>[2x]MGLLLPLALCILVLCCGAMSPPQLALNPSALLSRGCNDSDVLAVAGFALRDINKDRKDGYVLRLNRVNDAQEYRRGGLGSLFYLTLDVLETDCHVLRKKAWQDCGMRIFFESVYGQCKAIFYMNNPSRVLYLAAYNCTLRPVSKKKIYMTCPDCPSSIPTDSSNHQVLEAATESLAKYNNENTSKQYSLFKVTRASSQWVVGPSYFVEYLIKESPCTKSQASS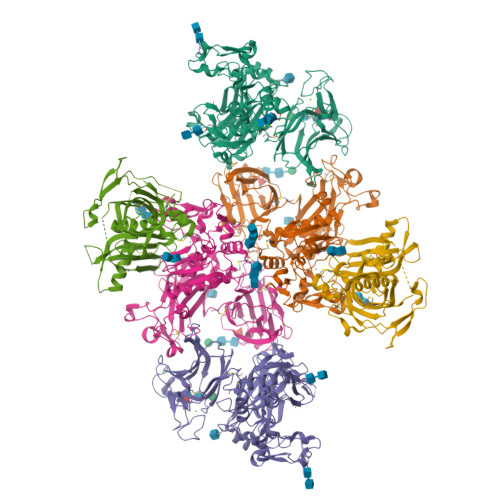CSLQSSDSVPVGLCKGSLTRTHWEKFVSVTCDFFESQAPATGSENSAVNQKPTNLPKVEESQQKNTPPTDSPSKAGPRGSVQYLPDLDDKNSQEKGPQEAFPVHLDLTTNPQGETLDISFLFLEPMEEKLVVLPFPKEKARTAECPGPAQNASPLVLPPHHHHHH;>WSHPQFEKVPIKYLPEENVHDADFGEQKDISEINLAAGLDLFQGDILLQKSRNGLRDPNTRWTFPIPYILADNLGLNAKGAILYAFEMFRLKSCVDFKPYEGESSYIIFQQFDGCWSEVGDQHVGQNISIGQGCAYKAIIEHEILHALGFYHEQSRTDRDDYVNIWWDQILSGYQHNFDTYDDSLITDLNTPYDYESLMHYQPFSFNKNASVPTITAKIPEFNSIIGQRLDFSAIDLERLNRMYNCTTTHTLLDHCTFEKANICGMIQGTRDDTDWAHQDSAQAGEVDHTLLGQCTGAGYFMQFSTSSGSAEEAALLESRILYPKRKQQCLQFFYKMTGSPSDRLVVWVRRDDSTGNVRKLVKVQTFQGDDDHNWKIAHVVLKEEQKFRYLFQGTKGDPQNSTGGIYLDDITLTETPCPTGVWTVRNFSQVLENTSKGDKLQSPRFYNSEGYGFGVTLYPNSRESSGYLRLAFHVCSGENDAILEWPVENRQVIITILDQEPDVRNRMSSSMVFTTSKSHTSPAINDTVIWDRPSRVGTYHTDCNCFRSIDLGWSGFISHQMLKRRSFLKNDDLIIFVDFEDITHLS[4x]NICOTINAMIDE-(6-DEAMINO-6-HYDROXY-ADENINE)-DINUCLEOTIDE 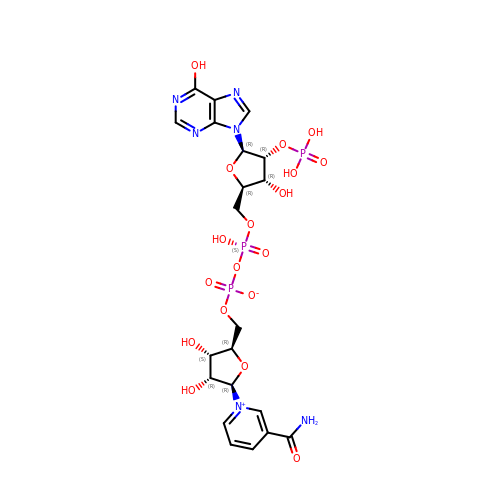PHOSPHATE | C21 H27 N6 O18 P3 | WKSUSMNNBQFESD-NNYOXOHSSA-N>[6x]MFEARLVQGSILKKVLEALKDLINEACWDISSSGVNLQSMDSSHVSL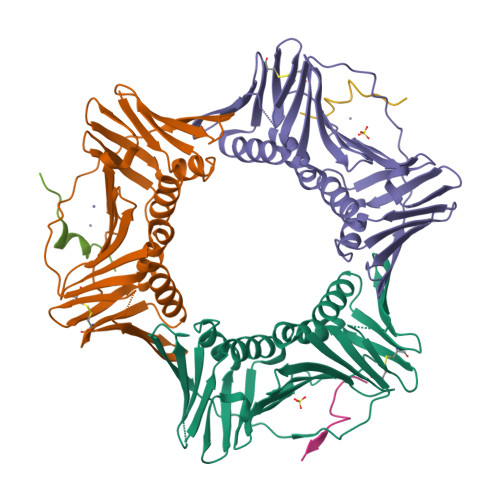VQLTLRSEGFDTYRCDRNLAMGVNLTSMSKILKCAGNEDIITLRAEDNADTLALVFEAPNQEKVSDYEMKLMDLDVEQLGIPEQEYSCVVKMPSGEFARICRDLSHIGDAVVISCAKDGVKFSASGELGNGNIKLSQTSNVDKEEEAVTIEMNEPVQLTFALRYLNFFTKATPLSSTVTLSMSADVPLVVEYKIADMGHLKYYLAPKIEDEEGS;>PKHTLDIFFKPLTH[6x]> MVNTIYIARHGYRSNWLPEGPYPDPLTGIDSDVPLAEHGVQQAKELAHYLLSLDNQPEAAFASPFYRCLETVQPIAKLLEIPVYLERGIGEWYRPDRKPVIPVPAGYEILSKFFPGVISQEWDSTLTPNEKGETEQEMYMRFKKFWPLFIERVEKEYPNVECILLVTHAASKIALGMSLLGYDNPRMSLNENGDKIRSGSCSLDKYEILKKSYDTIDETDDQTSFTYIPFSDRKWVLTMNGNTEFLSSGEEM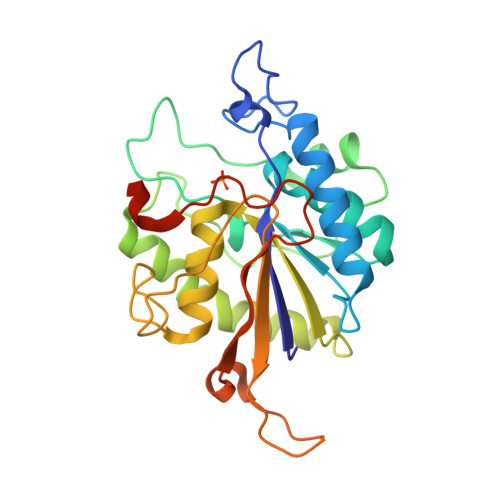NWNFDCVAEAGSDADIKKR Staphylococcus aureus pathogenicity islands (SaPIs) are molecular parasites that hijack helper phages for their transfer. SaPIbov5, the prototypical member of a family of cos type SaPIs, redirects the assembly of ϕ12 helper capsids from prolate to isometric. This size and shape shift is dependent on the SaPIbov5-encoded protein Ccm, a homolog of the ϕ12 capsid protein (CP). All tailed bacteriophages (order Caudovirales) package their genomes into preformed procapsids made from capsid protein (CP), with a ring-like portal protein (PP) forming a unique vertex at one end of the capsid.

An icosahedral reconstruction of the procapsids from 28,566 particle images reached a resolution of 4.0 Å (FSC = 0.143). 3D classification of the data without the application of symmetry (C1) indicated that only ≈1% of the shells had portals incorporated, and no further attempts to reconstruct in C1 or C5 were therefore made. These procapsids show the expected T = 4 organization with hexamer/pentamer clustering, and at this resolution secondary structure elements and many side chains were clearly visible, sufficient to model with confidence the proteins that make up the capsid. Cycles of manual model building and real-space refinement demonstrated conclusively that the pentamers (subunit A) were made of Ccm while the hexamers (subunits B–D) were composed of CP. One striking difference is the exceptionally long, extended N-arm in CP, especially in subunit B, where the chain could be traced all the way from the δ domain cleavage site at residue 129. The Ccm N-arm is rotated by ≈80° relative to CP around a pivot centered on CP residue L163, and folds behind the P-domain where it points towards the interior of the shell. Other major differences include the E-loops; unusually, both proteins have an α-helix within their E-loops, but the location of the helix is on opposite sides of the E-loop hairpin in the two proteins. In contrast, intercapsomeric interactions are sparse and mostly mediated through the P-domains, which interact around the icosahedral threefold axes (formed by three C subunits) and the quasi-threefold axes formed by A, B, and D subunits between two hexamers and a pentamer. At the icosahedral threefold axis, the N-arms from three B subunits come together to form a triskelion-like structure. Our results suggest a model for size redirection in which preferential incorporation of Ccm pentamers prevents the cylindrical midsection from forming by imposing a constant curvature on the capsid shell assembly.

> MKIMKEFKEQFGYQLSNFDDMDIKGYANLYQKDIGKDVSMIEQGLKQLSITETEVLLPEQINKKLLGVLNMNEVNQSSNTWVGTLTKQLVSSENNFNIQELPTARKEVFKELLVNRELPQTLRDVITITDDEHVESIPALSYIKDKLATNGIELSLNGSSKYFDRREGHIYTEVADSVVHGSDRTLDDLLKEIFINECVSYETTLLLDKNNASGLIDKDNQDLSLYNQGIKEVSNTSMYDGIKQAMKDIPQTFRRKVSVVMNTEHHDKLIKELAQMGLGTLAGDLTKLFNVSHVVVTDDAQDIFVGDFGHAIYAKYEPIMYNKKKQALKGVYQFALNYVFDIKIVPELLRIVKVK;>MRNFKNDNELLGGNEMPTLYELKQSLGMIGQQLKNKNDELSQKATDPNIDMEDIKQLETEKAGLQQRFNIVERQVQDIEEKEKAKVKDKGEAYQSLSDNEKMVKAKAEFYRHAILPNEFEKPSMEAQRLLHALPTGNDSGGDKLLPKTLSKEIVSEPFAKNQLREKARLTNIKGLEIPRVSYTLDDDDFITDVETAKELKAKGDTVKFTTNKFKVFAAISDTVIHGSDVDLVNWVENALQSGLAAKERKDALAVSPKSGLEHMSFYNGSVKEVEGADMYDAIINALADLHEDYRDNATIYMRYADYVKIISVLSNGTTNFFDTPAEKVFGKPVVFTDAAVKPIVGDFNYFGINYDGTTYDTDKDVKKGEYLFVLTAWYDQQRTLDSAFRIAKAKENTGPLPS[3x]> XRYSRLQLLLL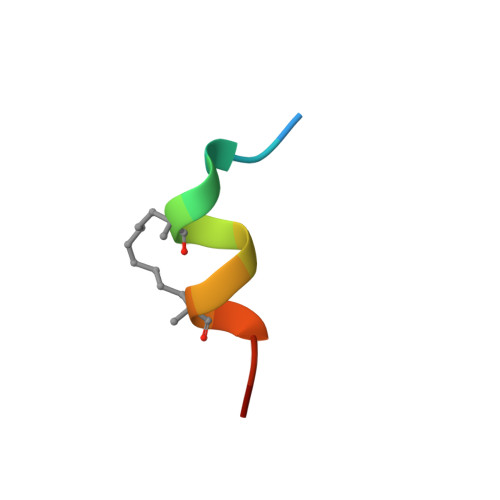FRX> ATITQDTPINQIFTDTALAEKMKTVLGKTNVTDTVSQTDLDQVTTLQADRLGIKSIDGVEYLNNLTQINFSNNQLTDITPLKNLTKLVDILMNNNQIADITPLANLTNLTGLTLFNNQITDIDPLKNLTNLNRLELSSNTISDISALSGLTSLQQLNFGNQVTDLKPLANLTTLERLDISSNKVSDISVLAKLTNLESLIATNNQISDITPLGILTNLDELSLNGNQLKDIGTLASLTNLTDLDLANNQISNLAPLSGLTKLTELKLGANQISNISPLAGLTALTNLELNENQLEDISPISNLKNLTYLTLYFNNISDISPVSSLTKLQRLFFSNNKVSDVSSLANLTNINWLSAGHNQISDLTPLANLTRITQLGLNDQAWTNAPVNYKANVSIPNTVKNVTGALIAPA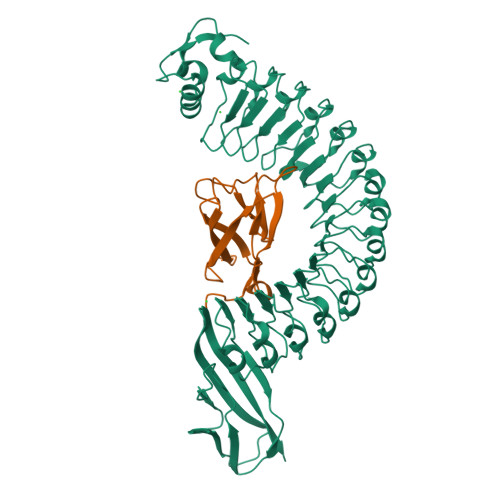TISDGGSYTEPDITWNLPSYTNEVSYTFSQPVTIGKGTTTFSGTVTQPLKA;> GPLGSWVIPPISCPENEKGEFPKNLVQIKSNRDKETKVFYSITGQGADKPPVGVFIIERETGWLKVTQPLDREAIAKYILYSHAVSSNGNAVEDPMEIVITVTDA6-[(2R)-2-(fluoromethyl)-3-hydroxy-propyl]-1,5-dimethyl-pyrimidine-2,4-dione | C10 H15 F N2 O3 | 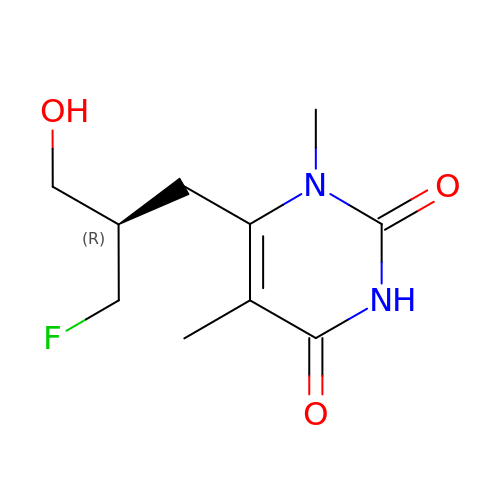OHXHFKXQCMBBKV-ZETCQYMHSA-N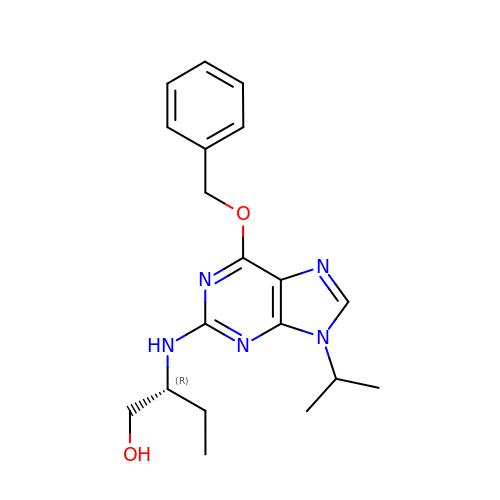(2R)-2-{[6-(BENZYLOXY)-9-ISOPROPYL-9H-PURIN-2-YL]AMINO}BUTAN-1-OL | C19 H25 N5 O2 | HGADNQLEUZSUEJ-OAHLLOKOSA-N> DPMDRWVGKTAVVTGASSGIGAAICVELANAGINVVGVARRTGPIEELKTQVKGKG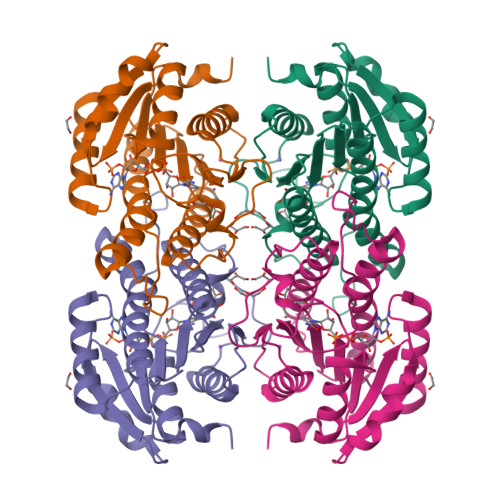SITARQCDVSSPEAVAETFKWIDDNLGCVHIMVNNAGIFTQGGITDVGGDMISEKDIMSVIDINLKGPILCSRHAIASMTRNKFDGHIVNINSIAGHYVPWSSKFNVYASSKYGLTGFSASLLNELADHKNKIKVTSVSPGLVRTAMTVAADDSEMPALTPKDVADAVLYVISTPPTVNINELTITPVTERRL>MSKPQPIAAANWKCNGSQQSLSELIDLFNSTSINHDVQCVVASTFVHLAMTKERLSHPKFVIAAQNAIAKSGAFTGEVSLPILKDFGVNWIVLGHSERRAYYGETNEIVADKVAAAVASGFMVIACIGETLQERESGRTAVVVLTQIAAIAKKLKKADWAKVVIAYEPVWAAGTGKVATPQQAQEAHALIRSWVSS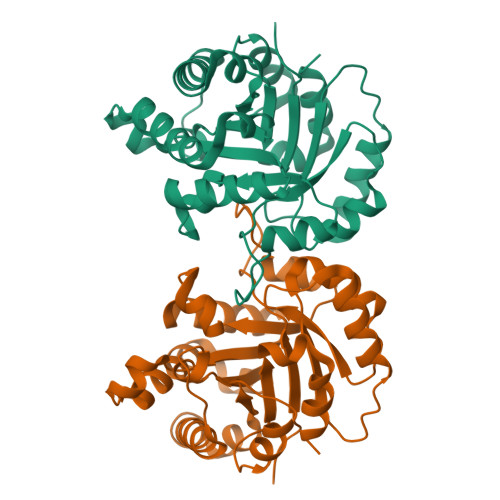KIGADVAGELRILYGGSVNGKNARTLYQQRDVNGFAVGGASLKPEFVDIIKATQ[4x]>MSQSNRELVVDFLSYKLSQKGYSWSQFSDVEENRTEAPEGTESEAVKQALREAGDEFELRYRRAFSDLTSQLHITPGTAYQSFEQVVNELFRDGVNWGRIVAFFSFGGALCVESVDKEMQVLVSRIAAWMATYLNDHLEPWIQENGGWDTFVELYGNNAAAESRKGQERLEGGMAVPPTYADLGKSARDVFTKGYGFGLGGHHHHHH[2x]

VDAC1 is a porin composed of a 19-strand β-barrel and an N-terminal α-helix (VDAC1-N) attached to the inside of the pore. In addition to its role in mitochondrial metabolite transport, VDAC1 has also been implicated as a key player in programmed cell death. Here, using cryo-EM and NMR we show that VDAC1 oligomerization or confinement in small lipid nanodiscs triggers the exposure of its N-terminal α-helix (VDAC1-N) which becomes available for partner protein binding. Biochemical assays demonstrate that VDAC1-N exhibits a pro-apoptotic function by promoting pore formation of the executor Bcl2 protein Bak via neutralization of BclxL.

To ensure that the VDAC1-N peptide remains stably bound to BclxL, we produced a single-chain construct where VDAC1-N (1–26) is fused to the C-terminus of BclxLΔLT (lacking its flexible loop and the transmembrane helix after residue 209). This construct allowed for crystal formation of suitable quality for a high-resolution structure determination by X-ray diffraction. The general binding mode between BclxL and VDAC1-N is reminiscent of BH3 peptides, e.g., as seen in the BclxL-Bak-BH3 complex. However, the binding site of VDAC1-N is shifted toward the periphery of the BclxL binding groove yet overlapping with the BH3 site. The C-terminal tail of VDAC1-N loosely binds to BclxL in an extended conformation, which is not seen for BH3 peptides. In our X-ray structure, VDAC1-N forms an amphipathic helix with the side chains of Leu10, Ser13, Asp16, Val17, and Phe18 facing the BclxL binding groove. To validate the structural model of the complex, we performed alanine scanning experiments where every individual residue in the binding region of VDAC1-N was mutated to alanine, followed by NMR-detected affinity measurements with each peptide. These experiments showed a strong impact of residues that participate in binding to BclxL, with the L10A mutation having the biggest impact (~20-fold reduction in affinity). Leu10 is the only large hydrophobic residue in VDAC1-N that is establishing a hydrophobic interaction with the BH3 binding groove in BclxL, thus markedly contributing to the overall binding affinity.>APITAPDITSICKDASSGIGNQEGAIRTRKCCPPSLGKKIKDFQFPNDKKVRMRWPAHKGTKKQVDDYRRA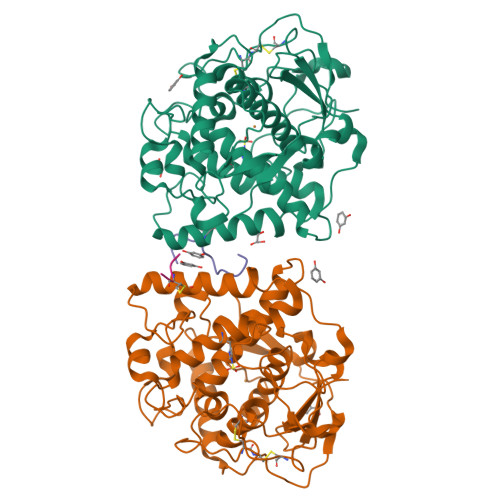IAAMRALPDDDPRSFVSQAKIHCAYCNGGYTQVDSGFPDIDIQIHNSWLFFPFHRWYLYFYERILGSLIDEPNFALPYWKWDEPKGMPISNIFLGDASNPLYDQYRDANHIEDRIVDLDYDGKDKDIPDQQQVACNLSTVYRDLVRNGVDPTSFFGGKYVAGDSPVANGDPSVGSVEAGSHTAVHRWVGDPTQPNNEDMGNFYSAGYDPVFYIHHANVDRMWKLWKELRLPGHVDITDPDWLNASYVFYDENKDLVRVYNKDCVNLDKLKYNFIENSKE[6x];>[6x]DGVFTTPCDPEYAGG>MRGSHHHHHHGSMDKNIIIGAMTALITPFKNGKVDEQSYARLIKRQIENGIDAVVPVGTTGESATLTHEEHRTCIEIAVETCKGTKVKVLAGAGSNATHDAVGLAKFAKEHGADGILSVAPYYNKPTQQGLYEHYKAIAQSVDIPVLLYNVPGRTGCEISTDTIIKLFRDCENIYGVKEASGNIDKCVDLLAHEPRMMLISGEDAINYPILSNGGKGVISVTSNLLPDMISALTHFALDENYKEAKKINDELYNINKILFCESNPIPIKTAMYLAGLIESLEFR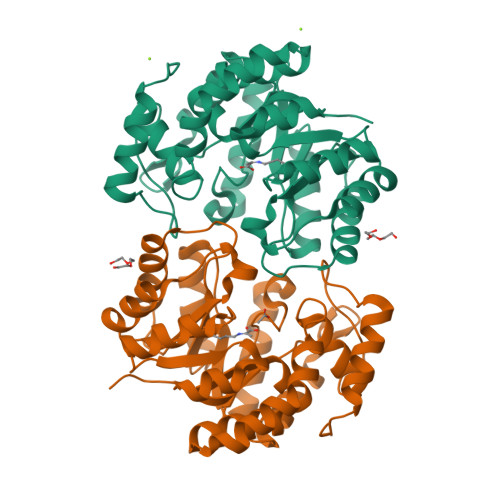LPLCSPSKENFAKIEEVMKKYKIKGF[6x]[[(2~{R},3~{S},4~{R},5~{R})-5-[2,4-bis(oxidanylidene)pyrimidin-1-yl]-3,4-bis(oxidanyl)oxolan-2-yl]methoxy-oxidanyl-phosphoryl] 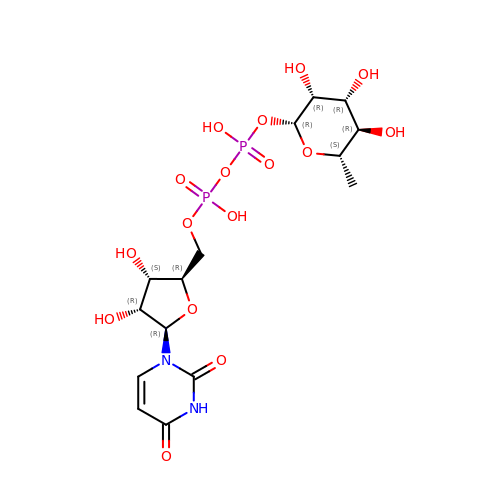[(2~{R},3~{R},4~{R},5~{R},6~{S})-6-methyl-3,4,5-tris(oxidanyl)oxan-2-yl] hydrogen phosphate | C15 H24 N2 O16 P2 | DRDCJEIZVLVWNC-SLBWPEPYSA-N>[4x]SHMKKLICISLYEDLSMTTYDLSKVDNAELIGIVENASEGTLFVFTCDRPNGSS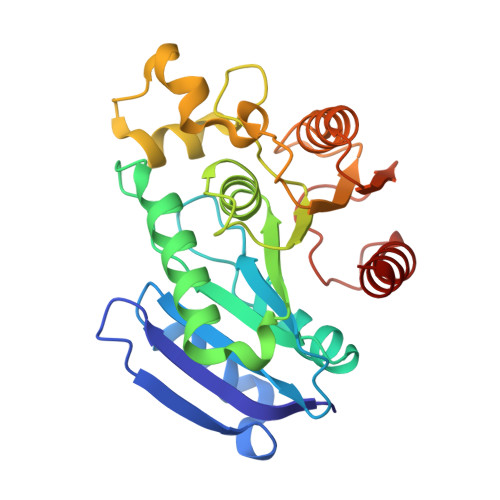VIMCPGGGFLKTNLENEGIDFAEWFTKLGITYIVFKYRMPHGNPDVPEQDTRLALKVVREKFPEFCDKLGVMGASIGGYLATFSATLLPDDEKPDFQILMYPVVSVDDRLTHFPCRERMFGHSYSPDKMEQYSPIEHITSGTPAAFIVAAADDAVVSPLNGIMYAARLQKADIPISLHIYPAGGHGFGYNDSFVYKQEWLQELGEWLAKL>[2x]GSHMPVVHVIDVESGNLQSLTNAIEHLGYEVQLVKSPKDFNISGTSRLILPGVGNYGHFVDNLFNRGFEKPIREYIESGKPIMGICVGLQALFAGSVESPKSTGLNYIDFKLSRFDDSEKPVPEIGWNSCIPSENLFFGLDPYKRYYFVHSFAAILNSEKKKNLENDGWKIAKAKYGSEEFIAAVNKNNIFATQFHPEKSGKAGLNVIENFLKQQSPPIPNYSAEEKELLMNDYSNYGLTRRIIACLDVRTNDQGDLVVTKGDQYDVREKSDGKGVRNLGKPVQLAQKYYQQGADEVTFLNITSFRD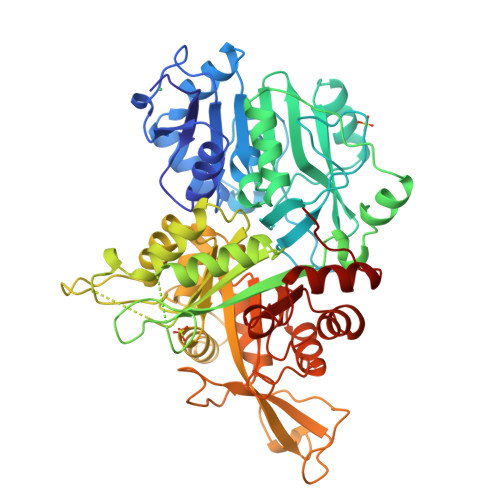CPLKDTPMLEVLKQAAKTVFVPLTVGGGIKDIVDVDGTKIPALEVASLYFRSGADKVSIGTDAVYAAEKYYELGNRGDGTSPIETISKAYGAQAVVISVDPKRVYVNSQADTKNKVFETEYPGPNGEKYCWYQCTIKGGRESRDLGVWELTRACEALGAGEILLNCIDKDGSNSGYDLELIEHVKDAVKIPVIASSGAGVPEHFEEAFLKTRADACLGAGMFHRGEFTVNDVKEYLLEHGLKVRMDEE> MDDISVIKNEDYEGSHRFLAEELLMPNANKTDGNRSTMFCSHLAQAVTLQKAEPPLVYTNFENQVGKYSTAG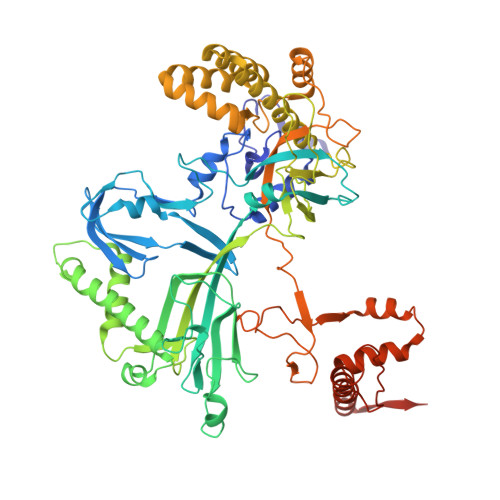YRKANSNYKVIEKIYKNDYNYVLIVQDQETGEYTLFERAECEFLTEHYGFQWDNDKIDSLKKDDTIEKDTVLYKNTCYDENMNFGYGVNLNAAYFSYKNETLEDAIVISESAAKKLGTFSVNKVKVSVNTNDILLNLYGDNENYKGFPDIGEHIKNQIIASRRRFDYNTALYELKNLNEMRDSDTPFFADGKIVDIEIFSNVPEEELKVQKYNEQVLYYINKQKEFSNNVYQKLKKIVEGKDNNVSDKLLHFYNNCKMRIDENISYTYQNSKFSGFIMEFTILEEEPLNKGSKITGRYGNKGVISKILPDDQMPTVAEGRFKGLKADICLNPLGVFNRLNPSQLIEQELNWIAKFIRKDMEEAGSNEEKVSILLDFLNRVNKEETELMEEFINSLNKTELEEFLNDIIENGIPICQKPFFGNIGLDELWELYNHYDHIDYFKCEGISTPLIIGEIYMVRLKHEPHSKFSARSTSFMNLRGLPAKSKNFKEHKDLYSKTPVRIGNMEISNLSLTNEMGSIMDMLNSYSNNETNRRELIMQLLTGNPFDTNIDLSDVESGTSKILKSLFTCLGLSIDDVEEEWENKLNGKVEDEK>MNAFDRARQSAIAAAREARGTYRNGLVTPTAGVAPGMTQANLIALPRDWAYDFLLYAQRNPKACPILDVSDAGSPTTLLAEGSDLRTDIPMYRIWRDGKLAEEVSDATQAWAEHDDMVAFLIGCSFTFET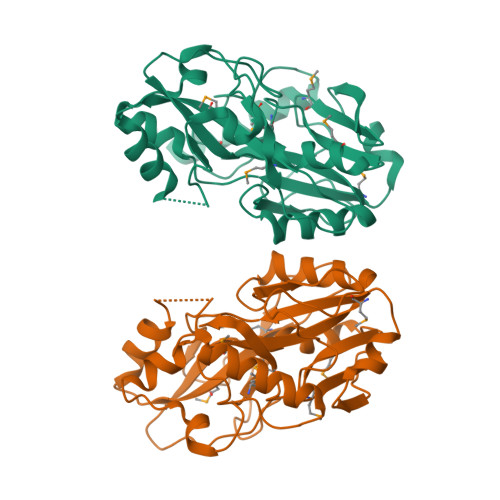PLQEAGIEVRHITDGCNVPMYRTNRACRPAGRLHGEMVVSMRPIPADRVAEASAISGRYPSVHGAPVHIGEPGRLGINDLSRPDFGDAVSIKPGEVPVFWACGVTPQAAVMASGVPFAITHSPGYMFITDVPDSTYHVLEHHHHHH[2x]> MNGDVQSVIRGYLERAQVAKTMSDAGRWNEAGDLLRQLMTDVKSCKISASNRDEHDARNTFLRALEANLKLVQQNVRDEDDLHEAMTRQSGSPEPPADPDVWSKPSPPLPSSSKFGATKKGVGAAGPRPREISKSTSSMSTNPADVKPANPTQGILPQNSAGDSFDASAYDAYIVQAVRGTMATNTENTMSLDDIIGMHDVKQVLHEAVTLPLLVPEFFQGLRSPWKAMVLAGPPGTGKTLIARAIASESSSTFFTVSSTDLSSKWRGDSEKIVRLLFELARFYAPSIIFIDQIDTLGGQRGNSGEHEASRRVKSEFLVQMDGSQNKFDSRRVFVLAATNIPWELDEALRRRFEKRIFIPLPDIDARKKLIEKSMEGTPKSDEINYDDLAARTEGFSGADVVSLCRTAAINVLRRYDTKSLRGGEL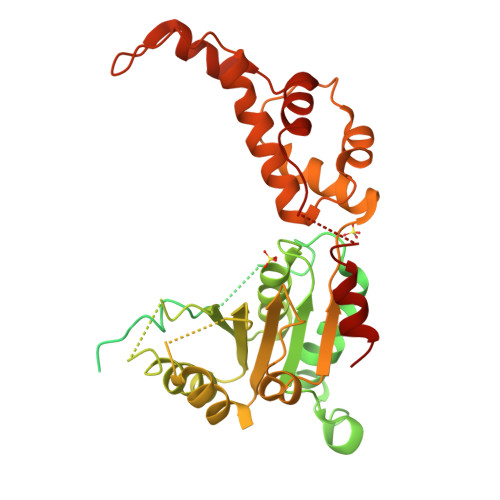TAAMESLKAELVRNIDFEAALQAVSPSAGPDTMLKCKEWCDSFGAM>SNAMKFLTVSDDMNFLRQVNTLVAGKGDMDSVIIGEGDAKGLGSKVLYRAKKGTPFDAVSEGILKIAGNYDYIAIGSTEVGREIAGYLSFKTGFYTATEI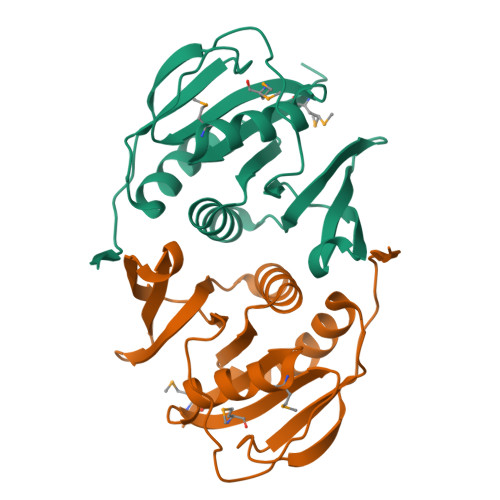FSLEFNGQKAHTKRFFYGGKTVIEEESDARILTVAPGVIEAKDLGTTPEIRDLEIGQSRIKITKFV[4x]>MRLELPVIPLRNTVILPHTTTPVDVGRAKSKRAVEEAMGADRLIFLVAQRDPEVDDPAPDDLYTWGVQAVVKQAMRLPDGTLQVMVEARARAQVTDYIPGPYLRARGEVFSEIFPIDEAVVRVLVEELKEAFEKYVANHKSLRLDRYQLEAVKGTSDPAMLADTIAYHATWTVAEKQEILELTDLEARLKKVLGLLSRDLERFELDKRVAQRVKEQMDTNQRESYLREQMKAIQKELGGEDGLSDLEALRKKIEEVGMPEAVKTKALKELDRLERMQQGSPEATVARTYLDWLTEVPWSKADPEVLDINHTRQVLDEDHYGLKDVKERILEYLAVRQLTQGLDVRNKAPILVLVGPPGVGKTSLGRSIARSMNRKFHRISLGGVRDEAEIRGHRRTYIGAMPGKLIHAMKQVGVINPVILLDEIDKMSSDWRGDPASAMLEVLDPEQNNTFTDHYLDVPYDLSKVFFITTANTLQTIPRPLLDRMEVIEIPGYTNMEKQAIARQYLWPKQVRESGMEGRIEVTDAAILRVISEYTREAGVRGLERELGKIARKGAKFWLEGAWEGLRTIDASDIPTYLGIPRYRPDKAETEPQVGTAQGLAWTPVGGTLLTIEVAAVPGSGKLSLTGQLGEVMKESAQAALTYLRAHTQDYGLPEDFYNKVDLHVHVPDGATPKDGPSAGITMATAIASALSRRPARMDIAMTGEVSLRGKVMPIGGVKEKLLAAHQAGIHKIVLPKDNEAQLEELPKEVLEGLEIKLVEDVGEVLEYLLLPEPTMPPVVQPSDNRQQPGAGA[6x]

The Lon protease is a AAA+ protein found in prokaryotes, archaea, and eukaryotic organelles. Lon is involved in cellular protein homeostasis by degrading damaged or misfolded abnormal proteins, which prevents these unwanted protein species from forming toxic aggregates. Lon is known to form a homohexamer; each protomer is composed of multiple domains, including an N-terminal substrate-binding globular domain (NGD), a long-helix domain (LH), a three-helix bundle (3H), a AAA+ ATPase module, and a protease domain. We show here, using cryo-electron microscopy (cryo-EM), that the activation process of the Lon AAA+ protease may involve a pentameric assembly and a substrate-dependent incorporation of the sixth protomer to form the substrate-pore-loop contacts seen in the translocating state.

To study the structure in the substrate-free state with ATPγS, we first set out to identify MtaLon with a point mutation in the N-terminal LH domain to eliminate substrate binding while preserving the native sequence of the AAA+ and the protease domains. Using a fluorescence polarization (FP) assay, we found that MtaLon-Y224S, which carries a mutation of the entry-gate residue Tyr224 to Ser19, does not interact with fluorescein isothiocyanate (FITC)-labeled casein. We conducted cryo-EM analysis on MtaLon-Y224S incubated with 5 mM of ATPγS (MtaLon-Y224S:ATPγS). Unexpectedly, both MtaLon-Y224S:ATPγS and wild-type MtaLon, whether with ADP or lacking nucleotide, predominantly formed left-handed spiral pentamers or spiral hexamers, rather than closed-ring hexamers. The substrate-free hexameric form also adopts a left-handed spiral structure. It is composed of the tethered pentamer and an additional Ac-protomer, Ac6*, which binds next to the protomer Ob1 and occupies the lowermost position of the spiral. Interestingly, the 3H subdomain of Ac6* occupies the axial cavity of the spiral complex and binds to the ATPase domains of the protomers 1–5, effectively blocking the accessibility of the pore loops and forming an inactive structure. In the absence of substrate, the sixth protomer binds to the pentamer, occupying the lowest position of the spiral oligomer, resulting in the formation of an auto-inhibited spiral hexamer.> MIVLFVDFDYFYAQVEE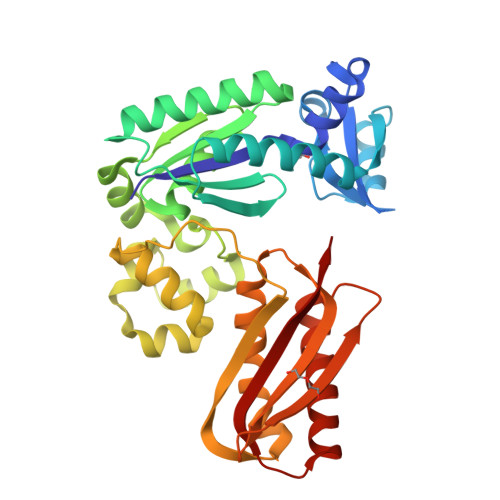VLNPSLKGKPVVVCVFSGRFEDSGAVATANYEARKFGVKAGIPIVEAKKILPNAVYLPMRKEVYQQVSSRIMNLLREYSEKIEIASIDEAYLDISDKVRDYREAYNLGLEIKNKILEKEKITVTVGISKNKVFAKIAADMAKPNGIKVIDDEEVKRLIRELDIADVPGIGNITAEKLKKLGINKLVDTLSIEFDKLKGMIGEAKAKYLISLARDEYNEPIRTRVRKSIGRIVTMKRNSRNLEEIKPYLFRAIEESYYKLDKRIPKAIHVVAVTEDLDIVSRGRTFPHGISKETAYSESVKLLQKILEEDERKIRRIGVRFSKFIT1-cyclohexyl-N-({6-fluoro-1-[2-(3-methoxyphenyl)pyridin-4-yl]-1H-indol-3-yl}methyl)methanamine 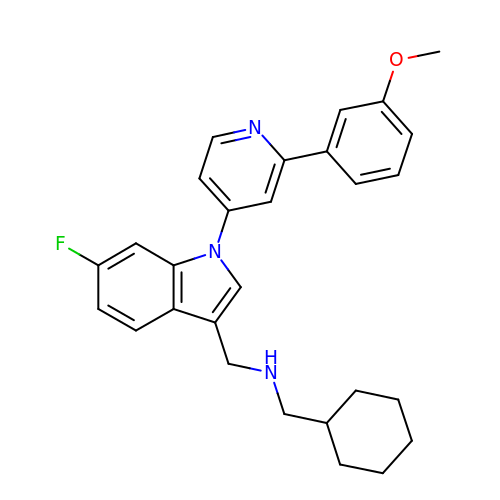| C28 H30 F N3 O | MDKNOMUATKMYAA-UHFFFAOYSA-N>MRLELPVIPLRNTVILPHTTTPVDVGRAKSKRAVEEAMGADRLIFLVAQRDPEVDDPAPDDLYTWGVQAVVKQAMRLPDGTLQVMVEARARAQVTDYIPGPYLRARGEVFSEIFPIDEAVVRVLVEELKEAFEKYVANHKSLRLDRYQLEAVKGTSDPAMLADTIAYHATWTVAEKQEILELTDLEARLKKVLGLLSRDLERFELDKRVAQRVKEQMDTNQRESYLREQMKAIQKELGGEDGLSDLEALRKKIEEVGMPEAVKTKALKELDRLERMQQGSPEATVARTYLDWLTEVPWSKADPEVLDINHTRQVLDEDHYGLKDVKERILEYLAVRQLTQGLDVRNKAPILVLVGPPGVGKTSLGRSIARSMNRKFHRISLGGVRDEAEIRGHRRTYIGAMPGKLIHAMKQVGVINPVILLDEIDKMSSDWRGDPASAMLEVLDPEQNNTFTDHYLDVPYDLSKVFFITTANTLQTIPRPLLDRMEVIEIPGYTNMEKQAIARQYLWPKQVRESGMEGRIEVTDAAILRVISEYTREAGVRGLERELGKIARKGAKFWLEGAWEGLRTIDASDIPTYLGIPRYRPDKAETEPQVGTAQGLAWTPVGGTLLTIEVAAVPGSGKLSLTGQLGEVMKESAQAALTYLRAHTQDYGLPEDFYNKVDLHVHVPDGATPKDGPSAGITMATAIASALSRRPARMDIAMTGEVSLRGKVMPIGGVKEKLLAAHQAGIHKIVLPKDNEAQLEELPKEVLEGLEIKLVEDVGEVLEYLLLPEPTMPPVVQPSDNRQQPGAGA[5x]

The Lon protease is a AAA+ protein found in prokaryotes, archaea, and eukaryotic organelles. Lon is involved in cellular protein homeostasis by degrading damaged or misfolded abnormal proteins, which prevents these unwanted protein species from forming toxic aggregates. Lon is known to form a homohexamer; each protomer is composed of multiple domains, including an N-terminal substrate-binding globular domain (NGD), a long-helix domain (LH), a three-helix bundle (3H), a AAA+ ATPase module, and a protease domain. We show here, using cryo-electron microscopy (cryo-EM), that the activation process of the Lon AAA+ protease may involve a pentameric assembly and a substrate-dependent incorporation of the sixth protomer to form the substrate-pore-loop contacts seen in the translocating state.

To study the structure in the substrate-free state with ATPγS, we first set out to identify MtaLon with a point mutation in the N-terminal LH domain to eliminate substrate binding while preserving the native sequence of the AAA+ and the protease domains. Using a fluorescence polarization (FP) assay, we found that MtaLon-Y224S, which carries a mutation of the entry-gate residue Tyr224 to Ser19, does not interact with fluorescein isothiocyanate (FITC)-labeled casein. We conducted cryo-EM analysis on MtaLon-Y224S incubated with 5 mM of ATPγS (MtaLon-Y224S:ATPγS). Unexpectedly, both MtaLon-Y224S:ATPγS and wild-type MtaLon, whether with ADP or lacking nucleotide, predominantly formed left-handed spiral pentamers or spiral hexamers, rather than closed-ring hexamers. Surprisingly, the pentameric form consistently emerged as the most prevalent class. The pentameric assembly forms a left-handed open-spiral structure. The open-spiral pentamer forms a large gap between the protomers Ob1 and Ob5. The pentamer forms a tensegrity helix triangle (THT), consisting of three overlapping LHs from Ob1, Ob3, and Ob5, forming an interlocked, letter A-shaped structure that tethers together five protomers.>[2x]ACDYTCGSNCYSSSDVSTAQAAGYKLHEDGETVGSNSYPHKYNNYEGFDFSVSS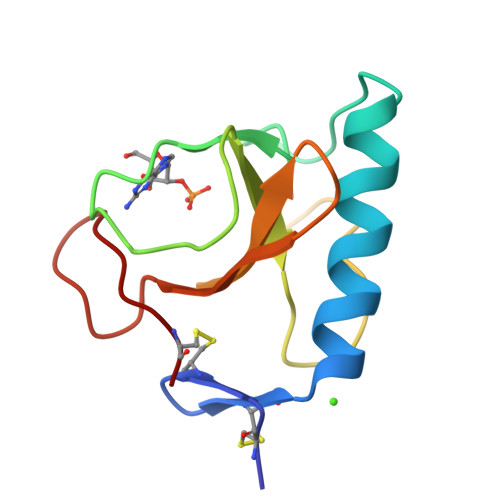PYYEWPILSSGDVYSGGSPGADRVVFNENNQLAGVITHTGASGNNAVECT>MNHYEVLVLGGGSGGITMAARMKRKVGAENVAIVEPSERHFYQPIWTLVGAGAKQLSSSGRPTASVIPSGVEWIKARVTELNPDKNCIHTDDDEKISYRYLIIALGIQLDYEKIKGLPEGFAHPKIGSNYSVKTVEKTWKALQDFKEGNAIFTFPNTPVKCAGAPQKIMYLSEAYFRKTGKRSKANIIFNTSLGAIFGVKKYADALQEIIQERNLTVNYKKNLIEVRADKQEAVFENLDKPGETQVISYEMLHVTPPMSPPDVLKTSPVADAAGWVDVDKETLQHRRYPNVFGIGDCTNLPTSKTAAAVAAQSGILDRTISVIMKNQTPTKKYDGYTSCPLVTGYNRV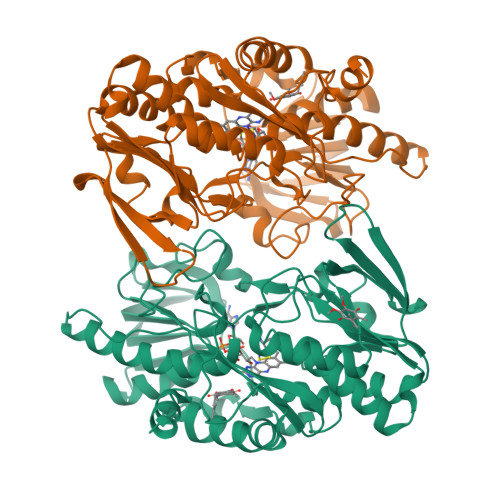ILAEFDYKAEPLETFPFDQSKERLSMYLMKADLMPFLYWNMMLRGYWGGPAFLRKLFHLGMSLEHHHHHH[2x]>[2x]SGLTPIHVAAFMGHLNIVLLLLQNGASPDVTNIRGETALHMAARAGQVEVVRCLLRNGALVDARAREEQTPLHIASRLGKTEIVQLLLQHMAHPDAATTNGYTPLHISAREGQVDVASVLLEAGAAHSLATKKGFTPLHVAAKYGSLDVAKLLLQRRAAADSAGKNGLTPLHVAAHYDNQKVALLLLEKGASPHATAKNGYTPLHIAAKKNQMQIASTLLNYGAETNIVTKQGVTPLHLASQEGHTDMVTLLLDKGANIHMSTKSGLTSLHLAAQEDKVNVADILTKHGADQDAHTKLGYTPLIVACHYGNVKMVNFLLKQGANVNAKTKNGYTPLHQAAQQGHTHIINVLLQHGAKPNATTANGNTALAIAKRLGYISVVDTLKVVTEEVTTTTTTITEKHKLNVPETMTEVLDVSDEEGDDTMTGDGGEYLRPEDLKELGDD

Ankyrins are a widely expressed scaffold protein family, which mainly function to link great varieties of functionally related but structurally diverse integral membrane proteins to the spectrin-based cytoskeletons. Each ankyrin contains an N-terminal membrane binding domain (MBD), which is composed of 24 ANK repeats and responsible for binding to diverse membrane targets. Following the MBD is an unstructured linker region of ~130 amino acid residues, followed sequentially by a ZU5-ZU5-UPA supramodule responsible for spectrin binding (SBD), a death domain (DD), and an intrinsically disordered C-terminal tail (CT) with varying lengths. We identified three distinct autoinhibitory segments from the intrinsically disordered linker and CT regions of AnkB, and elucidated the inhibition mechanism of these segments by detailed biochemical and structural investigations.

To ensure that we do not miss any possible residues forming the AI-c binding segment, we prepared a C-terminal 12 ANK repeats of AnkB followed by a 46-residue linker (aa 430–873), which covers a small part of AI-b, and solved the crystal structure of the protein at 1.95 Å resolution. The overall structure of our AnkB C-terminal 12 repeats-linker is very similar to that of AnkR_C12 (RMSD of 1.04 Å). However, our structure contains a longer linker folded back binding to the AnkB ANK repeats. A 20-residue linker (from Thr828 to Asp847 instead of 11 residues in AnkR_C12) is clearly defined, and this 20-residue linker extends to the repeat R18. Moreover, we observed a prominently positive-charged surface in the inner groove of R16-18 right next to Asp847, and the five residues following Asp847 are highly negatively charged and conserved (847DEEGDD852). We anticipate that this stretch of negatively charged residues is part of AI-c and involved in binding to MBD (likely R16-17 based on the length of the segment). In the AI-c folded-back structure, residues from AI-c form extensive hydrogen bonds with the residues in finger loops of ANK repeats. Perturbations of these hydrogen bonding interactions (e.g. the Asn834Lys substitution in AI-c or the Asn595Ala mutation in one of the ANK repeats finger loop) led to a few fold decreases in their bindings. Hydrophobic interactions also contribute to the AI-c autoinhibition. Met839 is buried in the hydrophobic pocket formed by Leu668 and Leu701; Leu843 interacts with sidechains of Leu597, Tyr630, and Ile635.> MNAPESVQAKPRKRYDAGVMKYKMGYWDGDYVPKDTDLLALFRITPQDGVDPVEAAAAVAGESSTATWTVVWTDRLTACDMYRAKAYRVDPVPNNPEQFFCYVAYDLSLFEEGSIANLTASIIGNVFSFKPIKAARLEDMRFPVAYVKTFAGPSTGIIVERERLDKFGRPLLGATTKPKLGLSGRNYGRVVYEGLKGGLDFMKDDENINSQPFMHWRDRFLFVMDAVNKASAATGEVKGSYLNV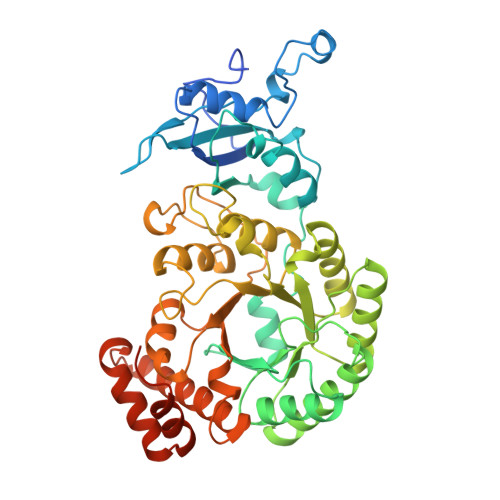TAGTMEEMYRRAEFAKSLGSVIIMVDLIVGWTCIQSMSNWCRQNDMILHLHRAGHGTYTRQKNHGVSFRVIAKWLRLAGVDHMHTGTAVGKLEGDPLTVQGYYNVCRDAYTQTDLTRGLFFDQDWASLRKVMPVASGGIHAGQMHQLIHLFGDDVVLQFGGGTIGHPQGIQAGATANRVALEAMVLARNEGRDILNEGPEILRDAARWCGPLRAALDTWGDISFNYTPTDTSDFAPTASVA>[4x]GSDHLFREQLARNYAFLGEE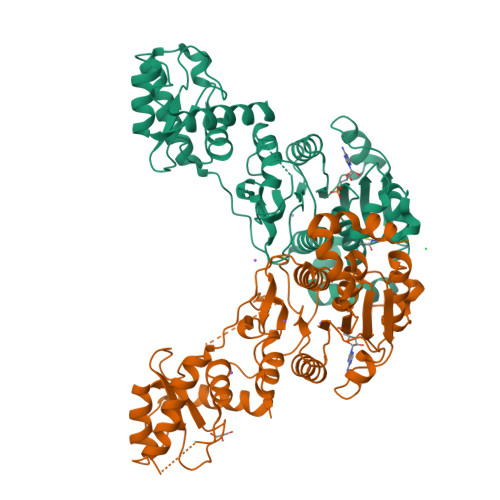GMRKIKEQYIVIVGAGEVGSWVCTMLIRSGCQKIMIIDPENISIDSLNTHCCAVLSDIGKPKVQCLKEHLSKIAPWSEIKARAKAWTKENSHDLIFADGESPTFIVDCLDNLESKVDLLEYAHHNKIDVISSMGVATKSDPTRVSINDISMTEFDPISRCVRRKLRKRGIATGISVVFSNEMLDPRRDDILSPIDCEHRAINAVRDEALRHLPELGTMPGIFGLSIATWILTKVSGYPMKENEVKNRLKFYDSILETFQKQMARLNENKERSSLLGLEEVGYIVEEMFRGKSPISGYSTKLALTKWEANKEISLTNVVLMTKEEQEIHEKRILLDGEKLTAVYSEEVLDFIERLFKEEEYYS> TRFTEEYQLFEELGKGAFSVVRR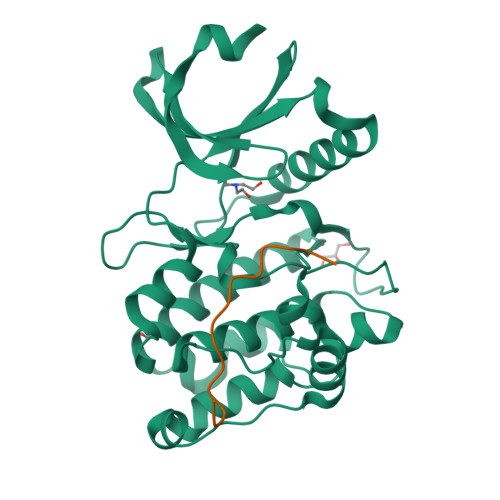CVKVLAGQEYAAKIINTKKLSARDHQKLEREARICRLLKHPNIVRLHDSISEEGHHYLIFDLVTGGELFEDIVAREYYSEADASHCIQQILEAVLHCHQMGVVHRNLKPENLLLASKLKGAAVKLADFGLAIEVEGEQQAWFGFAGTPGYLSPEVLRKDPYGKPVDLWACGVILYILLVGYPPFWDEDQHRLYKQIKAGAYDFPSPEWDTVTPEAKDLINKMLTINPSKRITAAEALKHPWISHR;> SKSRSTSSHGRRPLIRQDRIVG> 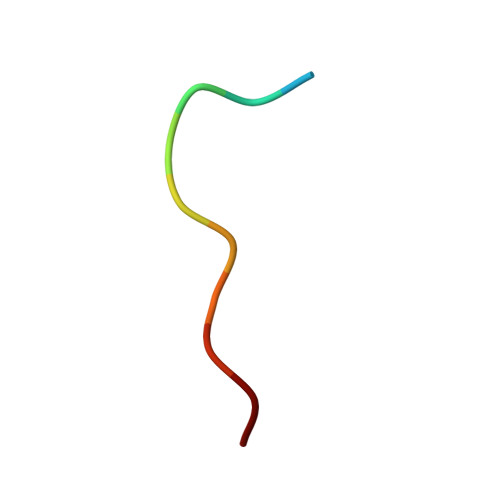XAPSYSPPPPP> IVGGYECKPYSQPHQVSLNSGYHFCGG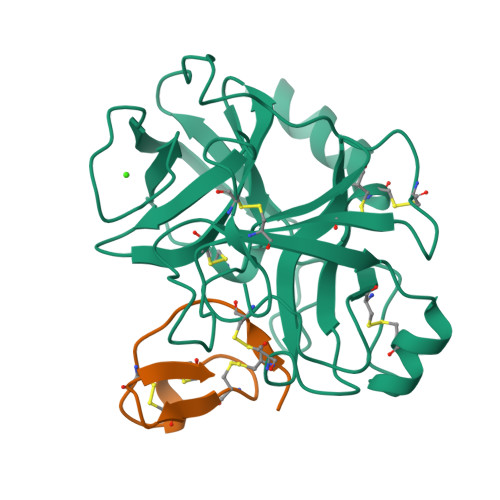SLVNENWVVSAAHCYKSRVEVRLGEHNIKVTEGSEQFISSSRVIRHPNYSSYNIDNDIMLIKLSKPATLNTYVQPVALPTSCAPAGTMCTVSGWGNTMSSTADSNKLQCLNIPILSYSDCNNSYPGMITNAMFCAGYLEGGKDSCQGDSGGPVVCNGELQGVVSWGYGCAEPGNPGVYAKVCIFNDWLTSTMASY;> RVCPRILMECKKDSDCLAECVCLEHGYCG>MEQIAQQQPQTLCIKHLAKNYSKRWVVKDVSFEMQSGQIVGLLGPNGAGKTTSFYMVVGLVRMDKGEIHLDNLDLSDLAMHERARKGIGYLPQEASIFRKLTIAENIMAILETRKDLNKQQRQQRLQELLNDFKITHIKDSLGMSVSGGERRRAEIARALAADPKFMLLDEPFAGVDPISVGDIKDIIRNLKDRGIGVLITDHNVRETLAICEHAYIVSEGAVIAEGSPQDILENEQVRKVYLGDDFTV[2x];> MIIRRYLVKQVVSTSLVVIALLTLIMMGGRLIKYFGVAAQGRLDAGVLFSIIGYRMPEFLTLILPLGFFIGLMLVFGRLYVDHEMAVLNGSGISRIRLGQLLIPLALVFLVIQGILMLWMTPWGLRQFDQLSSSQAVRTGFDLVRPKEFISSGPYTIYAGDLSEDRKNLKDIFFYQRAQKEGKPDVMILAKEATRVVMENETANVVDLIQGRRYEIYPGKAKYSQAEFQRYRLRLENDKSATFETDKVEALPSSKLWNKWNDPVIASEMGWRVFGPFTIVIALMMAVALCEVSPRQGRYYRLIPAIFIFASLIVLLIAIRTRISRDELGVWAYPAALAVYGIAAALFSRKQKLAPKIKKQIKRVRA;> MLARRIVAKHVTKTTALAMLGTTIVLVILQVLFTYLGELSNLKADYSAWQAFLYVLWGAPRYLYEILPISALIGAILGLGTLASNSELIVMRSVGISLWRIVGWVIRSALVLVLLSFALSEWVVPYTNERANSVKSHQSVAALGEVRGYWSREGQRFIYVDYANSQGQLKRIQVVDFDDNYRLKSVTNAEQGQFVKDGQWLLNHSQQMAIQGQGDAVLANAAKQPFSLALQPKYVHMVTIDPEDLSFSQLVSFMNYMREYSQVPKTYQLAFWKKVASPFALITLVLVACSFI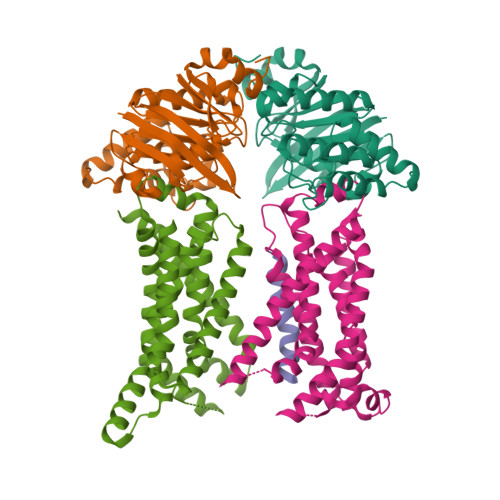FGPLRQQSMGFRLVIALFIGLGFYYLQDFLGYASLVYNPSPAWFVLGPIVLMFVAGSYLLYRAR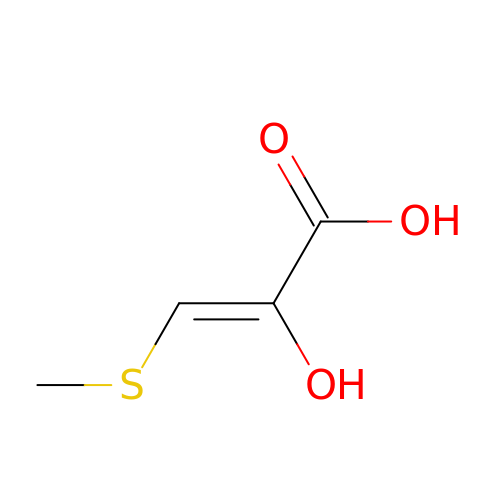(2Z)-2-hydroxy-3-(methylsulfanyl)prop-2-enoic acid | C4 H6 O3 S | VOKJWIQPUMADMU-IHWYPQMZSA-N> NSDVYAQEKQDFVQHFSQIVRVLTEDEMGHPEIGDAIARLKEVLEYNAIGGKYNRGLTVVVAFRELVEPRKQDADSLQRAWTVGWCVELLQAFFLVADDIMDSSLTRRGQICWYQKPGVGLDAINDANLLEACIYRLLKLYCREQPYYLNLIELFLQSSYQTEIGQTLDLL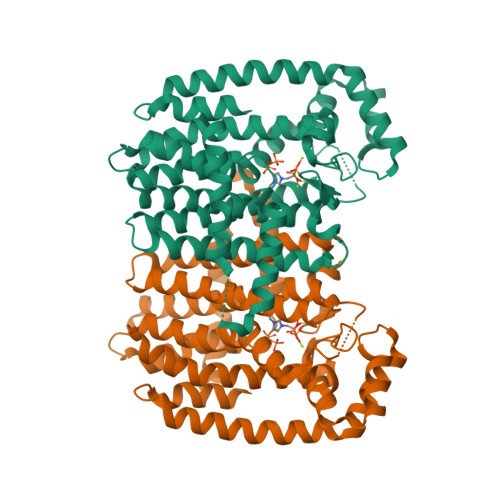TAPQGNVDLVRFTEKRYKSIVKYKTAFYSFYLPIAAAMYMAGIDGEKEHANAKKILLEMGEFFQIQDDYLDLFGDPSVTGKIGTDIQDNKCSWLVVQCLQRATPEQYQILKENYGQKEAEKVARVKALYEELDLPAVFLQYEEDSYSHIMALIEQYAAPLPPAVFLGLARKIYKRRK>[4x]GVKTFQFPFAEQLEKVAEQFPTFQILNEEGEVVNEEAMPELSDEQLKELMRRMVYTRILDQRSISLNRQGRLGFYAPTAGQEASQIASHFALEKEDFILPGYRDVPQIIWHGLPLYQAFLFSRGHFHGNQIPEGVNVLPPQIIIGAQYIQAAGVALGLKMRGKKAVAITYTGDGGTSQGNFYQGINFAGAFKAPAIFVVQNNRFAIS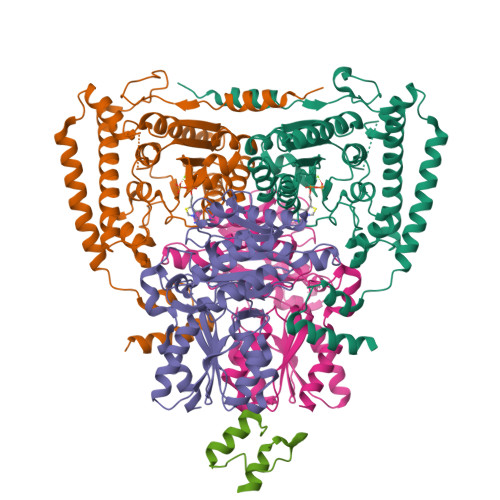TPVEKQTVAKTLAQKAVAAGIPGIQVDGMDPLAVYAAVKAARERAINGEGPTLIETLCFRYGPHTMSGDDPTRYRSKELENEWAKKDPLVRFRKFLEAKGLWSEEEENNVIEQAKEEIKEAIKKADETPKQKVTDLISIMFEELPFNLKEQYEIYKEKESK;>AQMTMVQAITDALRIELKNDPNVLIFGEDVGVNGGVFRATEGLQAEFGEDRVFDTPLAESGIGGLAIGLALQGFRPVPEIQFFGFVYEVMDSICGQMARIRYRTGGRYHMPITIRSPFGGGVHTPELHSDSLEGLVAQQPGLKVVIPSTPYDAKGLLISAIRDNDPVIFLEHLKLYRSFRQEVPEGEYTIPIGKADIKREGKDITIIAYGAMVHESLKAAAELEKEGISAEVVDLRTVQPLDIETIIGSVEKTGRAIVVQEAQRQAGIAANVVAEINERAILSLEAPVLRVAAPDTVYPFAQAESVWLPNFKDVIETAKKVMNF[4x];>[2x]AGPNRRVIAMPSVRKYAREKGVDIRLVQGTGKNGRVLKEDIDAFLAGGA>MGSDKIHHHHHHMELGIRDKGVLVLAASRGIGRAVADVLSQEGAEVTICARNEELLKRSGHRYVVCDLRKDLDLLFEKVKEVDILVLNAGGPKAGFFDELTNEDFKEAIDSLFLNMIKIVRNYLPAMKEKGWGRIVAITSFSVISPIENLYTSNSARMALTGFL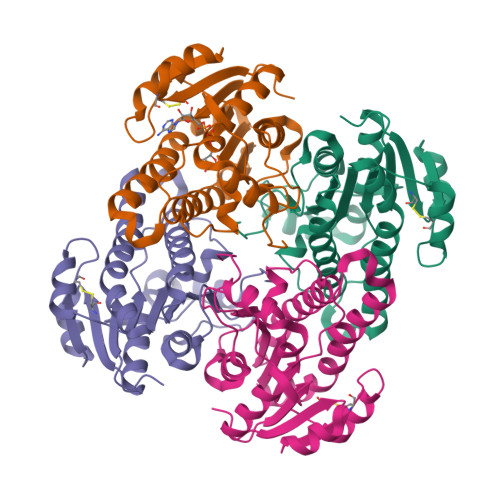KTLSFEVAPYGITVNCVAPGWTETERVKELLSEEKKKQVESQIPMRRMAKPEEIASVVAFLCSEKASYLTGQTIVVDGGLSKFPL[4x]>[4x]GPLGSPEFQVDMTFDVDTANNY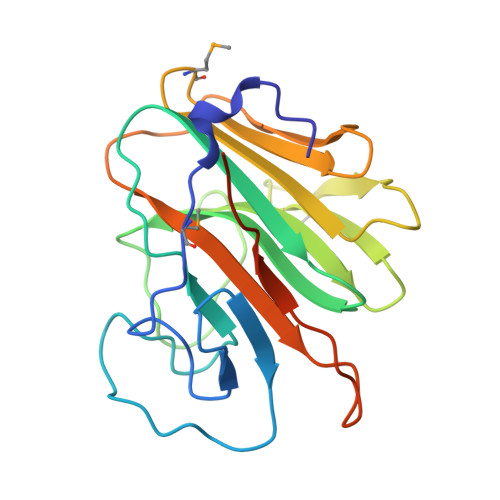LIISEDLRSFRSGDLSQNRKEQAERFDTALCVLGTPRFTSGRHYWEVDVGTSQVWDVGVCKESVNRQGKIELSSEHGFLTVGCREGKVFAASTVPMTPLWVSPQLHRVGIFLDVGMRSIAFYNVSDGCHIYTFIEIPVCEPWRPFFAHKRGSQDDQSILSICSVINPSAASAPVSSEGK>[2x]GPLGSMSLTPLCEDLPQFLQNYLPNAGQTENTIVPFVTLTYAQSLDARVSRGPGVRTTISHPETKTMTHYLRHHHDGILVGSGTVLADNPGLNCKWGPDPAANSPRPIIIDTKQKWRFDGSKMQELFIKRQGKPPIVVVTSEPIIKEQHVDYAICPINDTTKLVDWKKLFEILKEEFNIRSVMVEGGANVINQLLLRSDIVNSLIITIGSTFLGSSGTEVSPPQTVNLKDMSWWKGITDVVLCARLADD

Saccharomyces cerevisiae RIB7 (ScRIB7) is a potent target for anti-fungal agents because of its involvement in the riboflavin biosynthesis pathway as a NADPH-dependent reductase. In archaea and fungi, DAROPP is reduced at the phosphoribosyl moiety by RIB7 yielding 2, 5-diamino-6-ribitylamino-4(3H)-pyrimidinone 5′-phosphate (DARIPP), which is then deaminated into 5-amino-6-ribitylamino-2,4 (1H,3H)-pyrimidinedione 5′-phosphate (ARIPP) by RIB2. ScRIB7 exists as a stable homodimer, and each subunit consists of nine central β-sheets flanked by five helices, resembling the structure of RIB7 homologues. Here we report the crystal structure of Saccharomyces cerevisiae RIB7 at 2.10 Å resolution and its complex with NADPH at 2.35 Å resolution.

The structure of ScRIB7 was solved using single-wavelength anomalous dispersion (SAD). The crystals belong to space group P212121, with one asymmetric unit containing two ScRIB7 molecules. The RMSD between the C-alpha atoms of the two subunits is 0.3 Å. Each monomer is a mixed α/β structure: nine central β-strands flanked by five helices which are similar to those of the reductase domain of known RBSRs. The most likely dimeric interface was calculated using PISA, and the two molecules per asymmetric unit were modeled in the appropriate positions calculated by PISA. The size of the calculated interaction area was 1,303 Å2. The two subunit interfaces are made up of the four β-sheets (β1, β7–β9) and several loops (Lβ7–β8, Lβ8–β9). There are nineteen hydrogen bonds, and seven salt bridges between the protein atoms across the interface and the extensive hydrophobic surface formed by residues Tyr36, Leu40, Ala42, Leu190, Leu199, Ile201, Ile203, Phe207, Leu208, Val215, Val221, Leu223, Met226, Trp228, Trp229, Ile232, Val235, and Leu237. ScRIB7 has a unique α1 compared to MjRIB7, while EcRibD and BsRibG have N-terminal deaminase domain. Electronic density of loops Lα2′-β3 and Lβ1–α2 in ScRIB7 are missing probably due to their flexibility.>[4x]LGASWHRPDKCCLGYQKR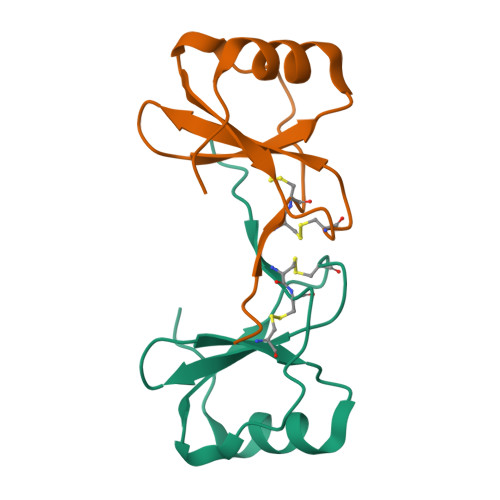PLPQVLLSSWYPTSQLCSKPGVIFLTKRGRQVCADKSKDWVKKLMQQLPVTAR>[2x]SNVPHKSSLPEGIRPGTVLRIRGLVPPNASRFHVNLLCGEEQGSDAALHFNPRLDTSEVVFNSKEQGSWGREERGPGVPFQRGQPFEVLIIASDDGFKAVVGDAQYHHFRHRLPLARVRLVEVGGDVQLDSVRIF

pmcHuman galectins (GAL) are oligomeric β-galactosidase-binding lectins assembled from small (∼15 kDa) protomeric carbohydrate recognition domains (CRD). Among prototype galectins, galectin-7 (GAL-7) is recognized for its preferential expression profiles in normal epithelial cells. For example, while extracellular GAL-7 can trigger apoptosis of activated T cells following binding to glycoreceptors via its GBS, it can also bind E-cadherin on epithelial cells independently of its GBS. In this work, we studied the impact of homodimer interface mutations on the induction of Jurkat T cell apoptosis, allowing us to positively and negatively modulate the biological activity of GAL-7 by designing a covalent disulfide bridge (G16C) and destabilizing mutation (G16S) to control homodimer strength, stability, and biological activity.

To examine whether these functional changes are rooted in structural perturbations at the molecular level, we solved the X-ray structures of lactose-bound WT GAL-7 and that of variants G16C and G16S in their apo and holo states. In contrast, our omit maps clearly show the presence of a bound lactose molecule in the GBS of both protomers within the WT, G16C, and G16S complexes. This is likely explained by the use of different crystallization techniques, i.e., soaking of WT GAL-7 crystals in lactose solution versus cocrystallization with lactose (present study). In a similar fashion, the ring opening of glucose was previously shown to be catalyzed by the amine group of a nearby lysine in the binding site of human serum albumin. Cα B′-factors between apo and holo WT structures show that chain B is less flexible, while chain A is more flexible in the presence of lactose. This indicates that loop 1 experiences distinct dynamic behavior in each GAL-7 chain upon ligand binding, an observation that was not immediately obvious from a previous GAL-7 dynamic investigation. In the presence of lactose, loop 5 Cα B′-factor values decrease in WT, while conversely increasing in G16X variants.> UCCCUG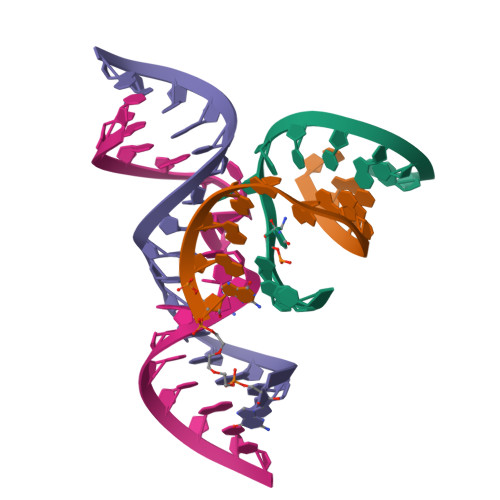UCCACCG;> CGGUGAGAAGGG;> GGCAGAGAAACACACGA;> UCGUGGUACAUUACCUGCC> YE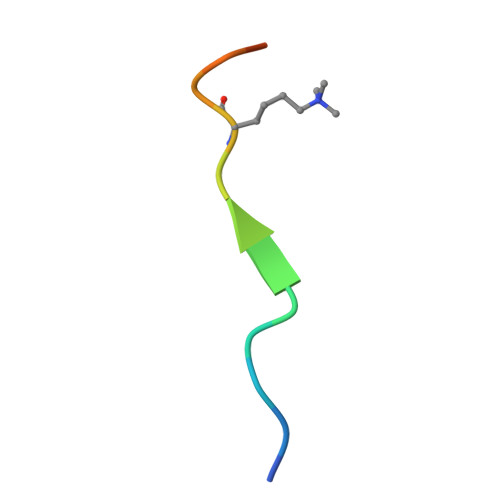PSTTARKVGRPGR> DLEPRFNNSSLKIEELQEALRKKEEEMKQMEERYKKYLEKAKSVIRTLDPKQNQGAAPEIQALKNQLQERDRLFHSLEKEYEKTKSQREMEEKYIVSAWYNMGMTLHKKAAEDRLASTGSGQSFLARQRQATSSRRSYPGHVQPA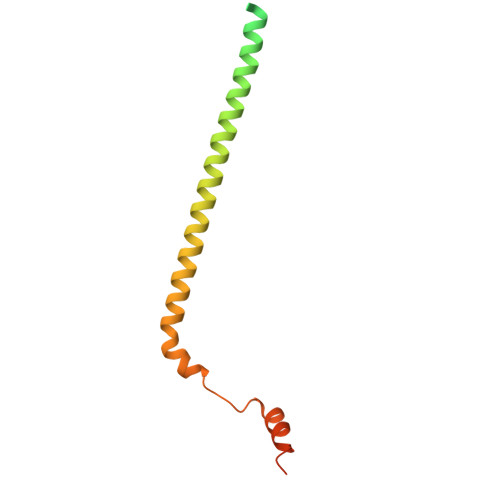TAR> MSAVGPGSNAGASVNGGSATAIATLLRNHKELKQRQGLFQAKQTDFFRYKRFVRALHSEEYANKSARQPEIYPTIPSNKIEDQLKSREIFIQLIKAQMVIPVKKLHSQECKEHGLKPSKDFPHLIVSNKAQLEADEYFVWNYNPRTYMDYLIVIGVVSIILALVCYPLWPRSMRRGSYYVSLGAFGILAGFFAVAILRLILYV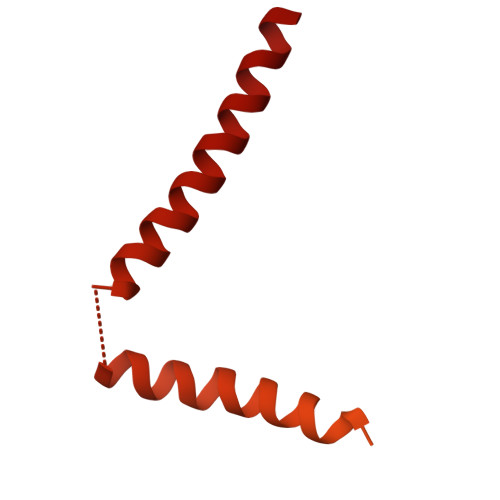LSLIVYKDVGGFWIFPNLFEDCGVLESFKPLYGFGEKDTYSYKKKLKRMKKKQAKRESNKKKAINEKAEQNXXXXXXXXXXXXXXXXXXXXXXXXXXXXXXXXXXXXXXXXXXXXXXXXXX> APLLLYANRRDLRLVDATNGKENATIVVGGLEDAAAVDFVFSHGLIYWSDVSEEAIKRTEFNKTESVQNVVVSGLLSPDGLACDWLGEKLYWTDSETNRIEVSNLDGSLRKVLFWQELDQPRAIALDPSSGFMYWTDWGEVPKIERAGMDGSSRFIIINSEIYWPNGLTLDYEEQKLYWADAKLNFIHKSNLDGTNRQAVVKGSLPHPFALTLFEDILYWTDWSTHSILACNKYTGEGLREIHSDIFSPMDIHAFSQQRQPNATNPCGIDNGGCSHLCLMSPVKPFYQCACPTGVKLLENGKTCKDGATELLLLARRTDLRRISLDTPDFTDIVLQLEDIRHAIAIDYDPVEGYIYWTDDEVRAIRRSFIDGSGSQFVVTAQIAHPDGIAVDWVARNLYWTDTGTDRIEVTRLNGTMRKILISEDLEEPRAIVLDPMVGYMYWTDWGEIPKIERAALDGSDRVVLVNTSLGWPNGLALDYDEGKIYWGDAKTDKIEVMNTDGTGRRVLVEDKIPHIFGFTLLGDYVYWTDWQRRSIERVHKRSAEREVIIDQLPDLMGLKATNVHRVIGSNPCAEENGGCSHLCLYRPQGLRCACPIGFELISDMKTCIVP;> EAFLLFSRRADIRRISLETNNNNVAIPLTGVKEASALDFDVTDNRIYWTDISLKTISRAFMNGSALEHVVEFGLDYPEGMAVDWLGKNLYWADTGTNRIEVSKLDGQHRQVLVWKDLDSPRALALDPAEGFMYWTEWGGKPKIDRAAMDGSERTTLVPNVGRANGLTIDYAKRRLYWTDLDTNLIESSNMLGLNREVIADDLPHPFGLTQYQDYIYWTDWSRRSIERANKTSGQNRTIIQGHLDYVMDILVFHSSRQSGWNECASSNGHCSHLCLAVPVGGFVCGCPAHYSLNADNRTCSAPTTFLLFSQKSAINRMVIDEQQSPDIILPIHSLRNVRAIDYDPLDKQLYWIDSRQNMIRKAQEDGSQGFTVVVSSVPSQNLEIQPYDLSIDIYSRYIYWTCEATNVINVTRLDGRSVGVVLKGEQDRPRAIVVNPEKGYMYFTNLQERSPKIERAALDGTEREVLFFSGLSKPIALALDSRLGKLFWADSDLRRIESSDLSGANRIVLEDSNILQPVGLTVFENWLYWIDKQQQMIEKIDMTGREGRTKVQARIAQLSDIHAVKELNLQEYRQHPCAQDNGGCSHICLVKGDGTTRCSCPMHLVLLQDELSCGEP;> KGQEGSVCLRSSDCASGLCCARHFWSKICKPVLKEGQVCTKHRRKGSHGLE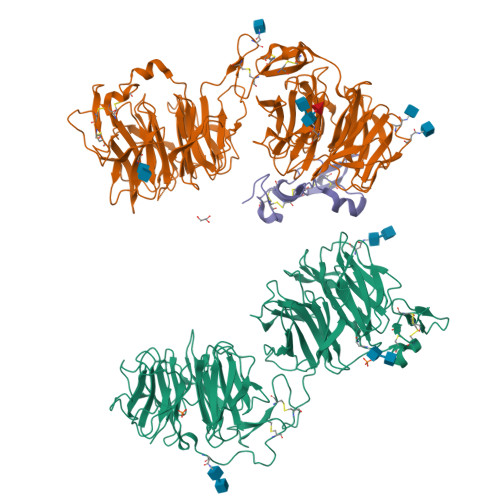IFQRCYCGEGLSCRIQKDHHQASNSSRLHTCQRH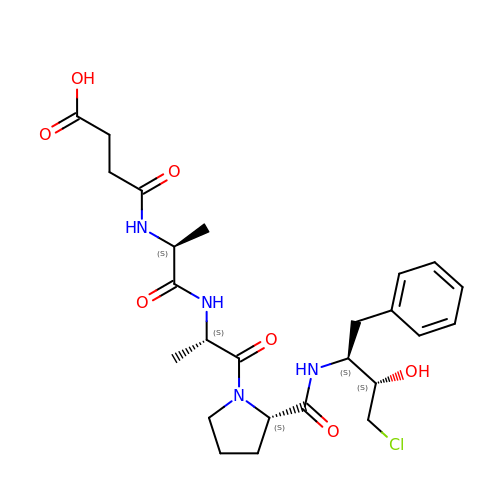N-(3-carboxypropanoyl)-L-alanyl-L-alanyl-N-[(2S,3S)-4-chloro-3-hydroxy-1-phenylbutan-2-yl]-L-prolinamide | C25 H35 Cl N4 O7 | NDDWTTUSJLUGKF-CZKCSJLSSA-N> AAQPPWPQGGQIEFRDFGLRYRP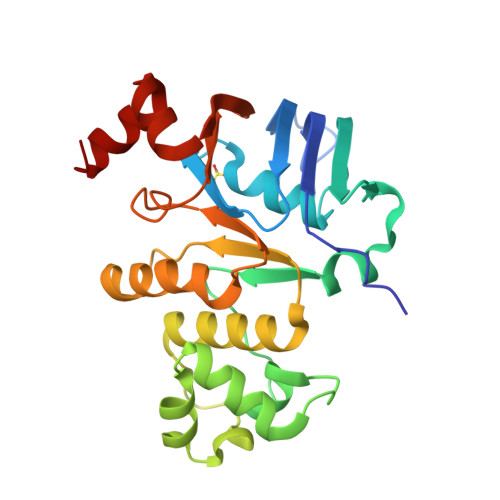ELPLAVQGVSFKIHAGEKVGIVGRTGAGKSSLASGLLRLQEAAEGGIWIDGVPIAHVGLHTLRSRISIIPQDPILFPGSLRMNLDLLQEHSDEAIWAALETVQLKALVASLPGQLQYKCADRGEDLSVGQKQLLCLARALLRKTQILILDEATAAVDPGTELQMQAMLGSWFAQCTVLLIAHDLRSVMDCARVLVMDKGQVAESGSPAQLLAQKGLFYRLAQESGLV>[2x]NYLMLNKSLCKVEGWVVVAKDNAIRFGESEQIIVTRE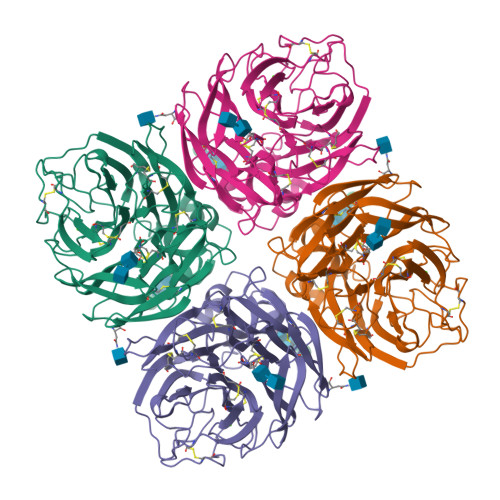PYVSCDPLGCKMYALHQGTTIRNKHSNGTIHDRTAFRGLISTPLGSPPIVSNSDFLCVGWSSTSCHDGIGRMTICVQGNNDNATATVYYDRRLTTTIKTWAGNILRTQESECVCHNGTCVVIMTDGSASSQAYTKVLYFHKGLVIKEEALKGSARHIEECSCYGHNSKVTCVCRDNWQGANRPVIEIDMNAMEHTSQYLCTGVLTDTSRPSDKSIGDCNNPITGSPGAPGVKGFGFLDSGNTWLGRTISPRSRSGFEMLKIPNAGTDPNSRITERQEIVDNNNWSGYSGSFIDYWDESSECYNPCFYVELIRGRPEEAKYVWWTSNSLVALCGSPVPVGSGSFPDGAQIQYFS>MSLRIGVIGTGKIGKEHINRITNKLSGAEIVAVTSVNQEAAQKVVEQYQLNATVYPNDDSLLADENVDAVLVTSWGPAHESSVLKAIKAQKYVFCEKPLATTAEGCMRIVEEEIKVGKRLVQVGFMRRYDSGYVQLKEALDNHVIGEPLMIHCAHRNPTVGDNYTTDMAVVDTLVHEIDVLHWLVNDDYESVQVIYPKKSKNALPHLKDPQIVVIETKGGIVINAEIYVNCKYGYDIQCEIVGEDGIIKL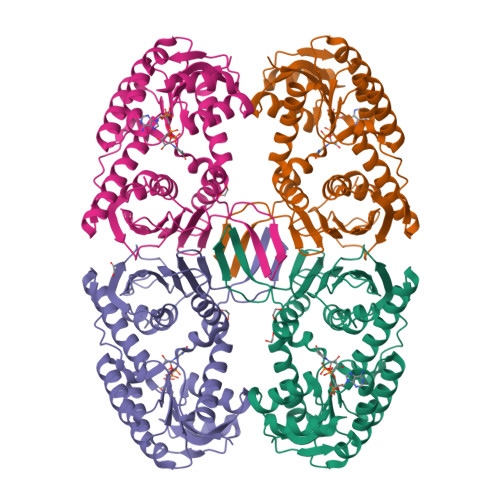PEPSSISLRKEGRFSTDILMDWQRRFVAAYDVEIQDFIDSIQKKGEVSGPTAWDGYIAAVTTDACVKAQESGQKEKVELKEKPEFYQ[4x]>[2x]MGSSHHHHHHSSENLYFQGHMTKSHSEEVIVPEFNSSAKELPRPLAEKCPSIIKKFISAYDAKPDFVARSPGRVNLIGEHIDYCDFSVLPLAIDFDMLCAVKVLNEKNPSITLINADPKFAQRKFDLPL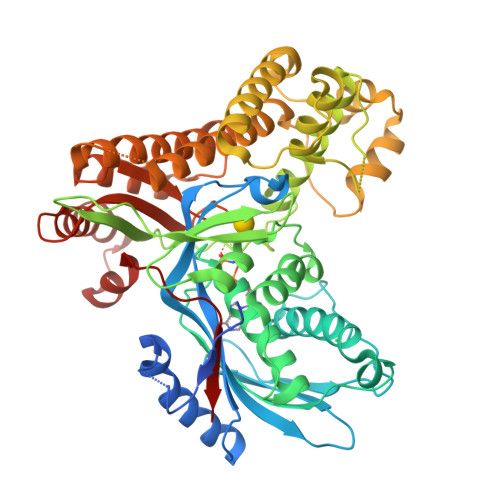DGSYVTIDPSVSDWSNYFKCGLHVAHSFLKKLAPERFASAPLAGLQVFCEGDVPTGSGLSSSAAFICAVALAVVKANMGPGYHMSKQNLMRITVVAEHYVGVNNGGMDQAASVCGEEDHALYVEFKPQLKATPFKFPQLKNHEISFVIANTLVVSNKFETAPTNYNLRVVEVTTAANVLAATYGVVLLSGKEGSSTNKGNLRDFMNVYYARYHNISTPWNGDIESGIERLTKMLVLVEESLANKKQGFSVDDVAQSLNCSREEFTRDYLTTSPVRFQVLKLYQRAKHVYSESLRVLKAVKLMTTASFTADEDFFKQFGALMNESQASCDKLYECSCPEIDKICSIALSNGSYGSRLTGAGWGGCTVHLVPGGPNGNIEKVKEALANEFYKVKYPKITDAELENAIIVSKPALGSCLYEL>MATHHTLWMGLALLGVLGDLQAAPEAQVSVQPNFQQDKFLGRWFSAGLASNSSWLREKKAALSMAKSVVAPATDGGLNLTSTFLRKNQCETRTMLLQPAGSLGSYSYRSPHWGSTYSVSVVETDYDQYALLYSQGSKGPGEDFRMATLYSRTQ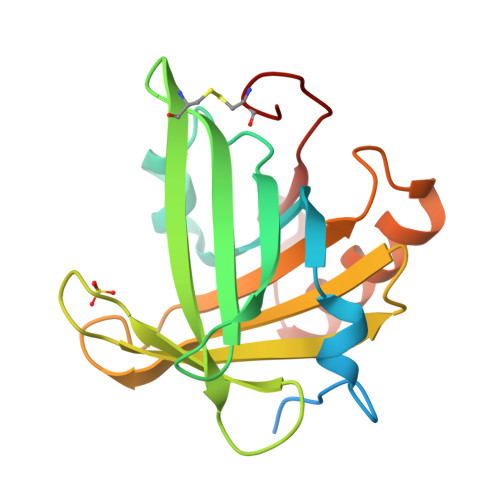TPRAELKEKFTAFCKAQGFTEDTIVFLPQTDKCMTEQ[2x]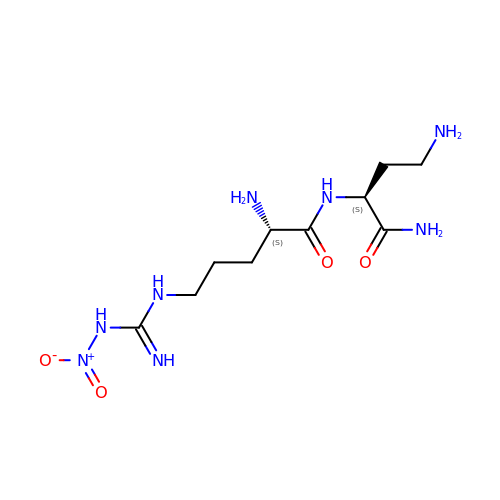L-N(OMEGA)-NITROARGININE-2,4-L-DIAMINOBUTYRIC AMIDE | C10 H22 N8 O4 | KUZKVXUOMSVPOA-BQBZGAKWSA-N>[2x]MEASVSFENGKIVVRLPITRPTSKIRVKKIENGVGIPVSTRKKSFPSDENLRDYYIEWQISFARDGKYDYELSRMVRLAHEHGILTYNDIYELLKFADDVKSYLEDKGIRRESTNEELYGFNIYEDVYPVAKKELPSGEFIGIVLKHAQRAVGYQSMVYVCIPLTNVEPSLAGRVARRNEVVKYEVPVDLMKELLKAFIIASETHKNDIVKFLRSIIGTS

R.PabI is a restriction DNA glycosylase that recognizes the sequence 5′-GTAC-3′ and hydrolyses the N-glycosidic bond of adenine in the recognition sequence. R.PabI from the hyperthermophilic archaeon Pyrococcus abyssi was the first HALFPIPE superfamily enzyme discovered. R.PabI recognizes the sequence 5′-GTAC-3′ of dsDNA at its electropositive HALFPIPE region and flips adenine and guanine bases in the recognition sequence to outside of the DNA helix using its β8-β9 loop. R.PabI hydrolyses the N-glycosidic bond of the flipped adenine using three catalytic residues (Y68, H211 and D214), Y68 is used to stabilize the catalytic water; H211 is used to localize the position of Y68; and D214 is used to stabilize the oxocarbenium ion intermediate and to deprotonate the catalytic water.

Here, we report the crystal structures of the R.PabI(Y68F-K154A) mutant in complex with three types of dsDNA. In this study, we determined the structures of R.PabI(Y68F-K154A) in complex with dsDNA(GTAC-3 bp-GTAC), dsDNA(GTAC-5 bp-GTAC) and dsDNA(nonspecific) at 2.45, 2.20 and 2.75 Å resolutions, respectively. In the R.PabI(Y68F-K154A)–dsDNA(GTAC-3 bp-GTAC) complex structure, structure models of amino acid residues 224–226 of chains A and B and those of amino acid residues 13–17 of chain B are not included in the final model due to low electron density. Although the DNA sequences used for cocrystallization are not identical, the structures of the R.PabI(Y68F-K154A)-dsDNA complexes are nearly identical; the maximal root mean square deviation (RMSD) among the complexes was 0.304 Å for 395 superposed Cα atoms in the asymmetric unit (between the dsDNA(GTAC-3 bp-GTAC) complex and the dsDNA(GTAC-5 bp-GTAC) complex). Because the side chain of T28 is inserted into the minor groove of dsDNA, the side chain hydroxyl group of T28 forms direct hydrogen bonds with the base and sugar groups of Thy−5 and Gua3′ in the dsDNA(GTAC-5 bp-GTAC) complex and with base groups of Gua-5 and Gua2′ in the dsDNA(GTAC-3 bp-GTAC) complex (DNA bases of the symmetrically related molecules are indicated by a prime). In the R.PabI(Y68F-K154A)–dsDNA(GTAC-5 bp-GTAC) complex and R.PabI(Y68F-K154A)–dsDNA(GTAC-3 bp-GTAC) complex structures, R.PabI dimers form 31 and 32 hydrogen bonds with the bound dsDNA structures, respectively. In fact, the roll angle at the base-stacking distorted region is larger in the dsDNA(GTAC-3 bp-GTAC) complex in which the TpA step (Thy-4 to Ade-3) exists at the distorted region. However, the structures of the R.PabI(Y68F-K154A)-dsDNA(GTAC-3 bp-GTAC) and R.PabI(Y68F-K154A)-dsDNA(GTAC-5 bp-GTAC) complexes show that R.PabI does not form any interactions with the R.PabI recognition sequence even if the sequence is located near the HALFPIPE region of the bound R.PabI dimer.>[4x]MKSKFKLTTAAAMLGLMVLAGGAQAQDKPREVLTGGHSVSAPQENRIYVMDSVFMHLTESRVHVYDYTNGKFLGMVPTAFNGHVQVSNDGKKIYTMTTYHERITRGKRSDVVEVWDADKLTFEKEISLPPKRVQGLNYDGLFRQTTDGKFIVLQNASPATSIGIVDVAKGDYVEDVTAAAGCWSVIPQPNRPRSFMTICGDGGLLTINLGEDGKVASQSRSKQMFSVKDDPIFIAPALDKDKAHFVSYYGNVYSADFSGDEVKVDGPWSLLNDEDKAKNWVPGGYNLVGLHRASGRMYVFMHPDGKEGTHKFPAAEIWVMDTKTKQRVARIPGRDALSMTIDQQRNLMLTLDGGNVNVYDISQPEPKLLRTIEGAAEASLQVQFHPVGGV;>AGGGGSSSGADHISLNPDLANEDEVNSCDYWRHCAVDGFLCSCCGGTTTTCPPGSTPSP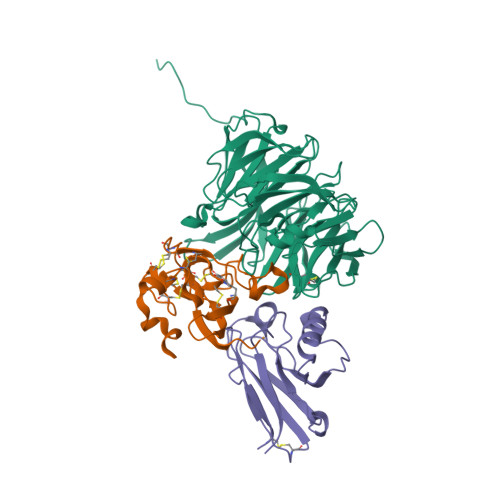ISWIGTCHNPHDGKDYLISYHDCCGKTACGRCQCNTQTRERPGYEFFLHNDVNWCMANENSTFHCTTSVLVGLAKN[4x];> ACDVSIEGNDSMQFNTKSIVVDKTCKEFTINLKHTGKLPKAAMGHNVVVSKKSDESAVATDGMKAGLNNDYVKAGDERVIAHTSVIGGGETDSVTFDVSKLKEGEDYAFFCSFPGHWSIMKGTIELGS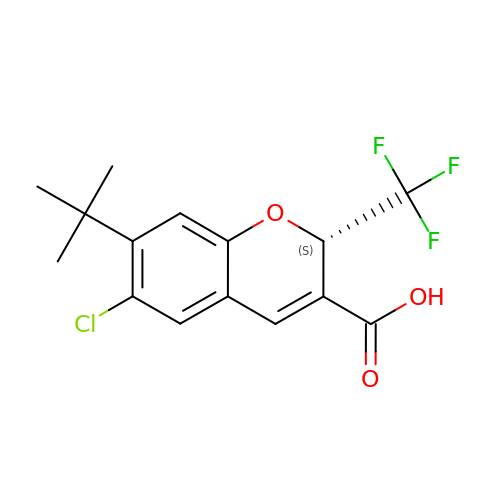(2S)-7-tert-butyl-6-chloro-2-(trifluoromethyl)-2H-chromene-3-carboxylic acid | C15 H14 Cl F3 O3 | QGCKNIAMHUUUDI-LBPRGKRZSA-N>[2x]MPREIITLQLGQCGNQIGFEFWKQLCAEHGISPEAIVEEFATEGTDRKDVFFYQADDEHYIPRAVLLDLEPRVIHSILNSPYAKLYNPENIYLSEHGGGAGNNWASGFSQGEKIHEDIFDIIDREADGSDSLEGFVLCHSIAGGTGSGLGSYLLERLNDRYPKKLVQTYSVFPNQDEMSDVVVQPYNSLLTLKRLTQNADCLVVLDNTALNRIATDRLHIQNPSFSQINQLVSTI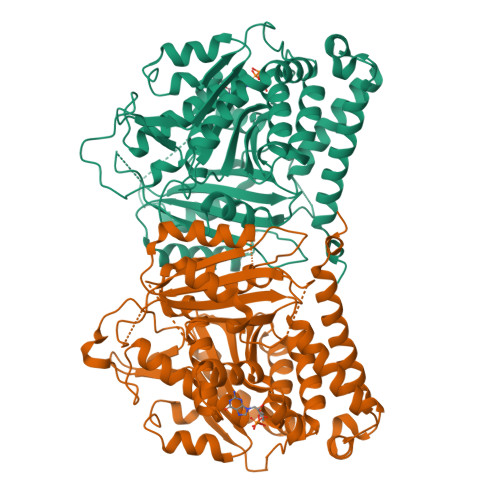MSASTTTLRYPGYMNNDLIGLIASLIPTPRLHFLMTGYTPLTTDQSVASVRKTTVLDVMRRLLQPKNVMVSTGRDRQTNHCYIAILNIIQGEVDPTQVHKSLQRIRERKLANFIPWGPASIQVALSRKSPYLPSAHRVSGLMMANHTSISSLFERTCRQYDKLRKREAFLEQFRKEDMFKDNFDEMDTSREIVQQLIDEYHAATRPDYISWGTQEQVDVDGGQKLISEEDLLLEHHHHHH>HHHHHHSSGLVPRGSHMSSVLKAYERFTLTQELQDQSEEGTIPPTTLKPVIRVFILTSNNPELRSRLLLFCLRIVLSNGARDSHRFGALLTMFSLPSATMLNHVKLADQSPEADIERVEIDGFEEGSFRLIPNARSGMSRGEINAYAALAEDLPDTLNHATPFVDSEVEGTAWDEIETFLDMCYSVLMQAWIVTCKCMTAPDQPAASIEKRLQKYRQQGRINPRYL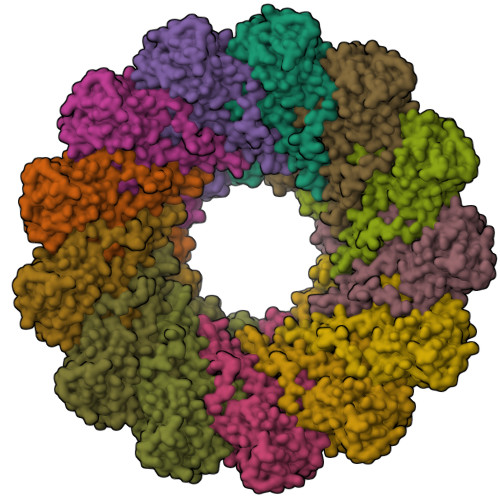LQPEARRIIQNVIRKGMVVRHFLTFELQLARAQSLVSNRYYAMVGDVGKYIENCGMGGFFLTLKYALGTRWPTLALAAFSGELTKLKSLMALYQTLGEQARYLALLESPHLMDFAAANYPLLYSYAMGIGYVLDVNMRNYAFSRSYMNKTYFQLGMETARKQQGAVDMRMAEDLGLTQAERTEMANTLAKLTTANRGADTRGGVNPFSSVTGTTQVPAAATGDTLESYMAADRLRQRYADAGTHDDEMPPLEEEEEDDTSAGPRTGPTLEQVALDIQNAAVGAPIHTDDLNAALGDLDI[13x]>[2x]MSSETVTLYEAIGGDATVRALTRRFY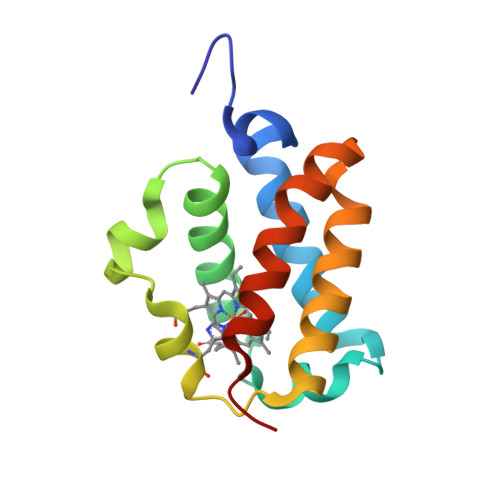ELMDTLPEAARCRAIHPADLSGSEAKFYDYLTGYLGGPPVYVEKHGHPMLRRRHFVAPIGPAERDEWLLCFRRAMDETIENAKLREIIWAPVERLAFHMQNQEADNP> MENTENSVDSKSIKNLEPKIIHGSESMDSGISLDNSYKMDYPEMGLCIIINNKNFHKSTGMTSRSGTDVDAANLRETFRNLKYEVRNKNDL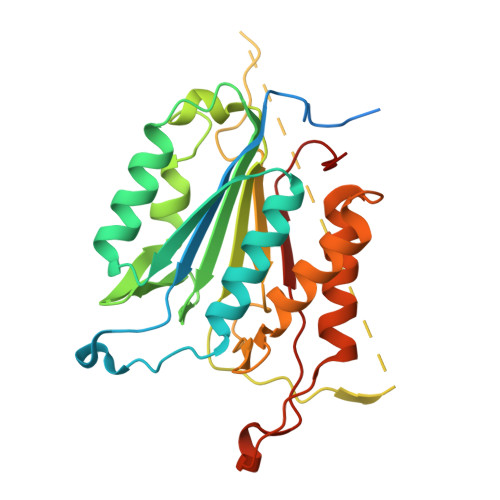TREEIVELMRDVSKEDHSKRSSFVCVLLSHGEEGIIFGTNGPVDLKKITNFFRGDRCRSLTGKPKLFIIQACRGTELDCGIETDSGVDDDMACHKIPVEADFLFAYSTAPGYYSWRNSKDGSWFIQSLCAMLKQYADKLEFMHILTRVNRKVATEFESFSFDATFHAKKQIPCIHSMLTKELYFYH2,3,4,6-tetra-O-sulfonato-alpha-D-glucopyranose | C6 H12 O18 S4 | 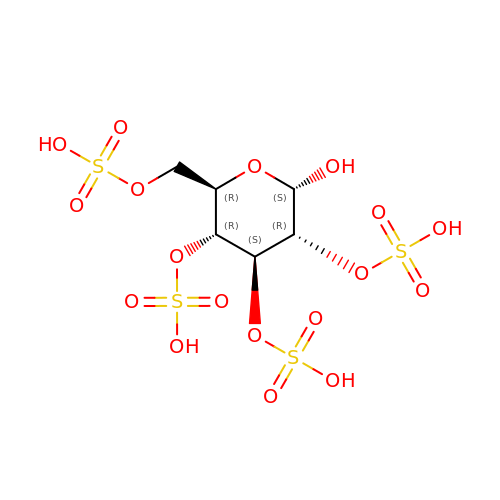SPIXVQOXHJQNTH-DVKNGEFBSA-N> AEIYNKDGNKVDLYGKAVGLHYFSKGNGENSYGGNGDMTYARLGFKGE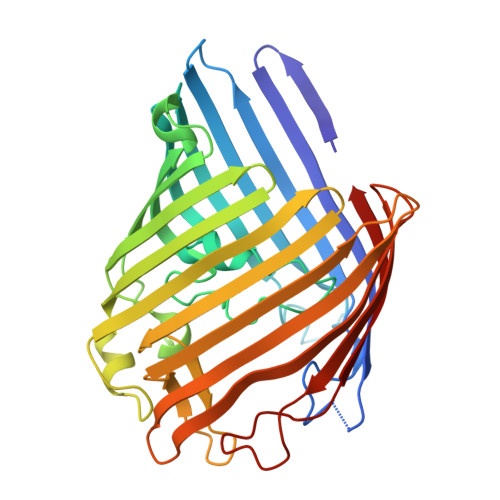TQINSDLTGYGQWEYNFQGNNSEGADAQTGNKTRLAFAGLKYADVGSFDYGRNYGVVYDALGYTDMLPEFGGDTAYSDDFFVGRVGGVATYRNSNFFGLVDGLNFAVQYLGKNERDTARRSNGDGVGGSISYEYEGFGIVGAYGAADRTNLQEAQPLGNGKKAEQWATGLKYDANNIYLAANYGETRNATPITNKFTNTSGFANKTQDVLLVAQYQFDFGLRPSIAYTKSKAKDVEGIGDVDLVNYFEVGATYYFNKNMSTYVDYIINQIDSDNKLGVGSDDTVAVGIVYQF>GSHMASMKKKGSVVIVGRINLSGDTAYAQQTRGEEGCQETSQTGRDKNQVEGEVQIVSTATQTFLATSINGVLWTVYHGAGTRTIASPKGPVTQMYTNVDKDLVGWQAPQGSRSLTPCTCGSSDLYLVTRHADVIPVRRRGDSRGSLLSPRPISYLKGSAGGPLLCPAGHAVGIFKAAVSTRGVAKA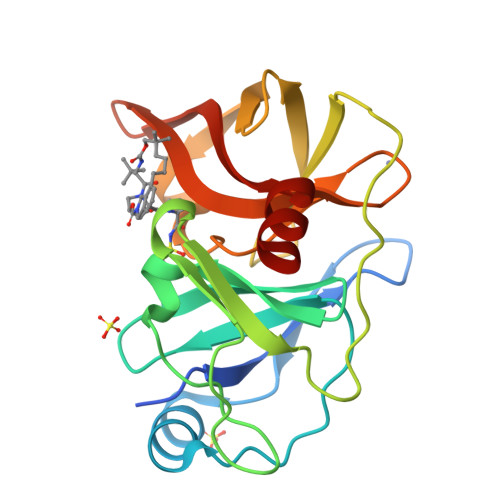VDFIPVESLETTMRSP[2x]>GGAUGGCCGCCUAUGGUCGUCAAAUAAACUACGAAAGUAGGAUAAAGUGGAAUAGUAAGGUUUAGCUAUUCUGCGGUUUCAUCUUGUAAAGAUGGAGCUUGAGUAGGCAAGUGAGAUAUCAAUUUUUCUUAGUAUGUGAGGGUAACACUUUAGCAGAGGAGAAAAGUUGACUGGGUCUUUGCAGAGAUUCAGUUGAGUUCGGAAGAGCAAUAAGAAUAACUCAUAGAAUUCAAUGCGAGAGGUAGGGAACUAAUCCCUCCCUAUAAUCGCGGUAUUCAAUAUGAUAGUUUACUUAACAUCAAAUUGGGGAAACCCUUUAAGAUAAGAUAGUGUACGGGUGGUGCCGUUAUUAUCCUUUGAUAGAGUGUACCAGCACCUAUCGAUGAAGUAAACUUGGAAUAUGGUGGUAGGGAUACCACAUCGGGUAGUUAAGUAUUCUGUCGUUCAAAAGGCGGCGGAGCUUGUGAUAGACCGCUACCUGAAACCACUGCAAAACCAAACUUAUAUUUGCAUUUAGGAUUGCAAAAUCAUAAAAAUCAAAAUAAGAAAAAGUGUCUAUCAGUUUUGACCGAAAGGUGUCUACAUAGUAAUGAGUUGUUCAUUGCCACAAACACUCUCAAGGUGAAUGUGAUUCUUUCGAAAGGUUUCUAACACCGCAAGUGUGAAUCUGCUCGGCAGGGUAGAAGAAAAUAAGUAAGAAGAGAGUAGGUUAAAACUCAAA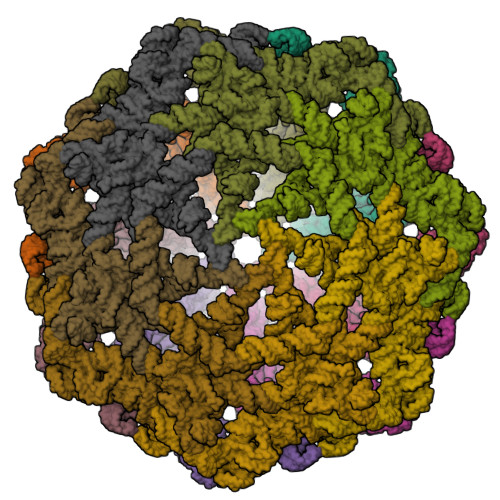GAGUGGUUCACUUAAAUAACCGACAUUGGUUGUUACAUCUCAAAAGGAUGUGGAAACAAAGGGAAUAGAUAAUCCUUUUAAAGACAACUACAAUAUGGUGUAUUCUCAGCCU[14x]N-[(1-methyl-1H-pyrazol-4-yl)methyl]furan-2-carboxamide | C10 H11 N3 O2 | 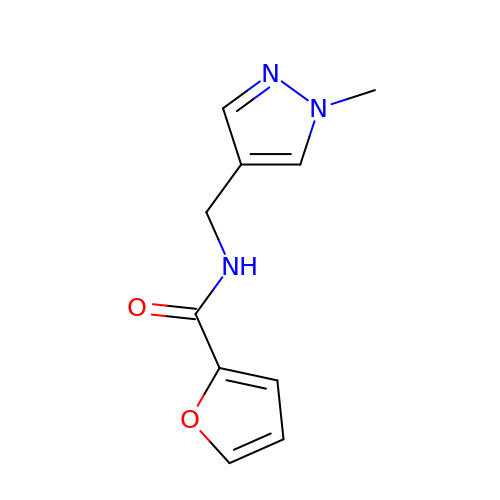ZPCCCCZFCHPBOS-UHFFFAOYSA-N> GASGSGTGSGSMSTLYLTQPDAVLSKKHEAFHVALKQEDGSWKKQPIPAQTLEDIVLLGYPSITGEALGYALELGLPVHYLTQFGKYVGSALPSESRNGQLRLAQFRAHEDPIQRLDIVKAFVKGKVHNQYNLLYRRGQVDNPLKGRGKLVMRQQTLEQVRGIEGLAAREYFASWQEMLGHEWTFTGRFRRPPTDPVNALLSFGYGLLRTQVTAA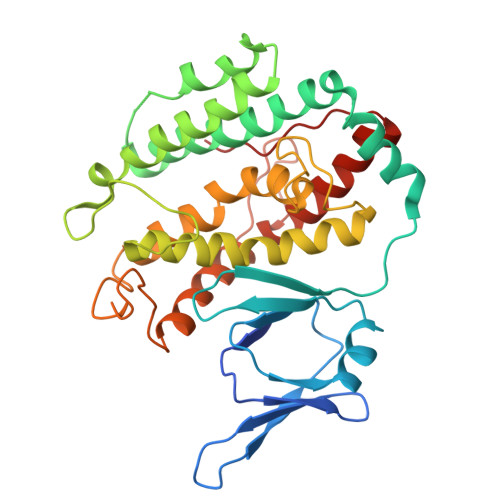VHIAGLDPYIGFLHETTRGQPAMILDLMEEFRALVADSVVLTVLKQREIQRQDFTESLGAFRLTDSATKTFLGAFDRKLSSEFKHPIFNYKCTYRRAIELQARLLARHLQEGVVYEPLVIR>MTDNNKYRDVEIRAPRGNKLTAKSWLT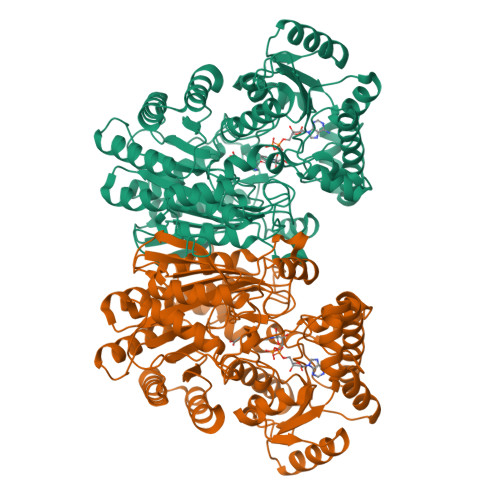EAPLRMLMNNLDPQVAENPKELVVYGGIGRAARNWECYDKIVETLTRLEDDETLLVQSGKPVGVFKTHSNAPRVLIANSNLVPHWANWEHFNELDAKGLAMYGQMTAGSWIYIGSQGIVQGTYETFVEAGRQHYGGSLKGKWVLTAGLGGMGGAQPLAATLAGACSLNIESQQSRIDFRLETRYVDEQATDLDDALVRIAKYTAEGKAISIALHGNAAEILPELVKRGVRPDMVTDQTSAHDPLNGYLPAGWTWEQYRDRAQTEPAAVVKAAKQSMAVHVQAMLDFQKQGVPTFDYGNNIRQMAKEEGVADAFDFPGFVPAYIRPLFCRGVGPFRWAALSGEAEDIYKTDAKVKELIPDDAHLHRWLDMARERISFQGLPARICWVGLGLRAKLGLAFNEMVRSGELSAPVVIGRDHLDSGSVSSPNAETEAMRDGSDAVSDWPLLNALLNTAGGATWVSLHHGGGVGMGFSQHSGMVIVCDGTDEAAERIARVLTNDPGTGVMRHADAGYDIAIDCAKEQGLDLPMITG[2x]>[2x]MIDLAIGQVPIANWVSSATDWITSTFSSGFDVIQKSGTVLMNGITGALTAVPFWLMIAVVTILAILVSGKKIAFPLFTFIGLSLIANQGLWSDLMSTITLVLLSSLLSIIIGVPLG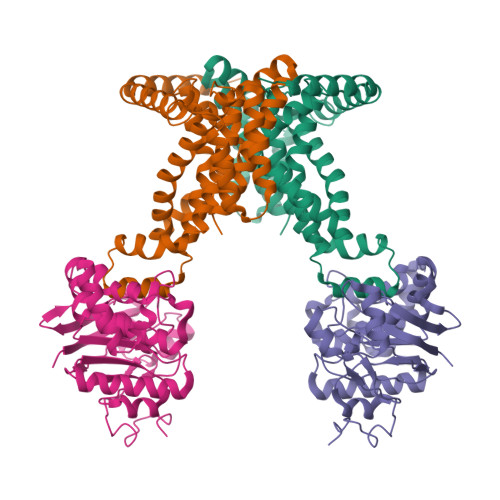IWMAKSDLVAKIVQPILDFMQTMPGFVYLIPAVAFFGIGVVPGVFASVIFALPPTVRMTNLGIRQVSTELVEAADSFGSTARQKLFKLEFPLAKGTIMAGVNQTIMLALSMVVIASMIGAPGLGRGVLAAVQSADIGKGFVSGISLVILAIIIDRFTQKLNVSPLEKQGNPTVKKWKRGIALVSLLALIIGAFSGMSFGKTASDKKVDLVYMNWDSEVASINVLTQAMKEHGFDVKTTALDNAVAWQTVANGQADGMVSAWLPNTHKTQWQKYGKSVDLLGPNLKGAKVGFVVPSYMNVNSIEDLTNQANKTITGIEPGAGVMAASEKTLNSYDNLKDWKLVPSSSGAMTVALGEAIKQHKDIVITGWSPHWMFNKYDLKYLADPKGTMGTSENINTIVRKGLKKENPEAYKVLDKFNWTTKDMEAVMLDIQNGKTPEEAAKNWIKDHQKEVDKWFKGSIEGRHHHHHH;>MAVKIKIEHLTKIFGKRIKTALTMVEKGEPKNEILKKTGATVGVYDTNFEINEGEIFVIMGLSGSGKSTLLRLLNRLIEPTSGKIFIDNQDVATLNKEDLLQVRRKTMSMVFQNFGLFPHRTILENTEYGLEVQNVPKEERRKRAEKALDNANLLDFKDQYPKQLSGGMQQRVGLARALANDPEILLMDEAFSALDPLIRREMQDELLELQAKFQKTIIFVSHDLNEALRIGDRIAIMKDGKIMQIGTGEEILTNPANDYVKTFVEDVDRAKVITAENIMIPALTTNIDVDGPSVALKKMKTEEVSSLMAVDKKRQFRGVVTSEQAIAARKNNQPLKDVMTTDVGTVSKEMLVRDILPIIYDAPTPLAVVDDNGFLKGVLIRGSVLEALADIPDEDEVEEIEKEEENK[2x]>MTKAVHTKHAPAAIGPYSQGIIVNNMFYSSGQIPLTPSGEMVNGDIKEQTHQVFSNLKAVLEEAGASFETVVKATVFIADMEQFAEVNE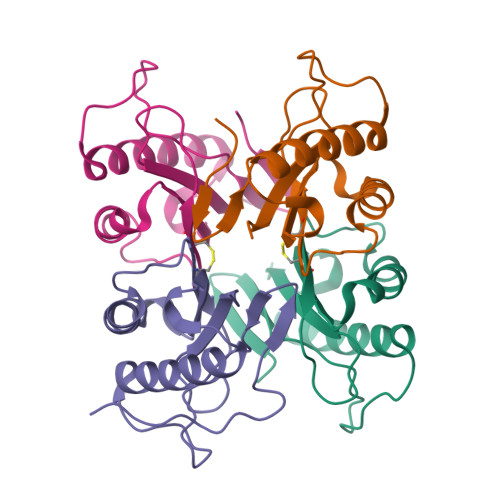VYGQYFDTHKPARFCVEVARLPKDALVEIEVIALVK[20x]> MARVAVLISGTGSNLQALIDSTREPNSSAQIDIVISNKAAVAGLDKAERAGIPTRVINHKLYKNRVEFDSAIDLVLEEFSIDIVCLAGFMRILSGPFVQKWNGKMLNIHPSLLPSFKGSNAHEQALETGVTVTGCTVHFVAEDVDAGQIILQEAVPVKRGDTVATLSERVKLAEHKIFPAALQLVASGTVQLGENGKICWVKEEHHHHHH

Interestingly, PMX is a multitargeted antifolate that also inhibits the folate-dependent reactions catalyzed by glycinamide ribonucleotide (GAR) formyltransferase (GARFTase) (in the trifunctional GARFTase/glycinamide ribonucleotide synthase (GARS)/aminoimidazole ribonucleotide synthetase (AIRS) enzyme) and 5-aminoimidazole-4-carboxamide ribonucleotide formyltransferase (AICARFTase) (in the bifunctional enzyme AICARFTase/inosine monophosphate cyclohydrolase (ATIC)) in de novo purine biosynthesis. Although all these antifolates are used clinically, their use is often associated with dose-limiting toxicities arising from the lack of tumor selectivity, as well as emergence of drug resistance. By metabolite rescue in KB cells and in vitro enzyme assays, de novo purine biosynthesis was identified as a targeted pathway (at 5-aminoimidazole-4-carboxamide ribonucleotide formyltransferase (AICARFTase) and glycinamide ribonucleotide formyltransferase (GARFTase)). To better understand the molecular effects of modifications to 6-substituted thieno[2,3-d]pyrimidine analogs on GARFTase inhibition, we determined the structures of select analogs (4, 5, 9, and 10) with a range of inhibitor potencies in complex with GARFTase and β-GAR substrate. The thieno[2,3-d]pyrimidine scaffold of all analogs makes polar contacts with the backbone atoms of Leu899, Glu948, and Asp951 in GARFTase.

Our in vitro results demonstrate that compound 9 is a uniquely potent inhibitor of human GARFTase. The most potent analog, 9 (0.17 μM), is a fluorinated thieno compound with the fluorine positioned to make an intramolecular contact with the amide hydrogen of the l-glutamate moiety (as predicted from NMR and molecular docking), thus restricting the side chain. The α-carboxylate of the l-glutamate of 9 is stabilized in the GARFTase active site by contacts with the side chain of Arg871, as well as the backbone amide of Ile898. Compound 9 is 882-fold more inhibitory toward GARFTase than the corresponding des-fluoro 11, indicating the importance of the fluorine for GARFTase inhibition in this structural motif. Compound 9 showed a Ki of 0.17 μM (17-, 25-, and 882-fold more potent than 2, 10, and 11, respectively). Compound 10, a nonfluorinated 3-C bridged thieno compound, is ∼25-fold less active than 9 in GARFTase inhibition and exhibits the same contacts between the l-glutamate and GARFTase as those seen for 9. This implies that fluorination in 9 relative to the closely related nonfluorinated compounds 10 and 11 may bias the conformation prior to binding GARFTase, thereby reducing its entropic penalty upon binding (i.e., leading to increased potency).>[2x]GIGDPVTCLKSGA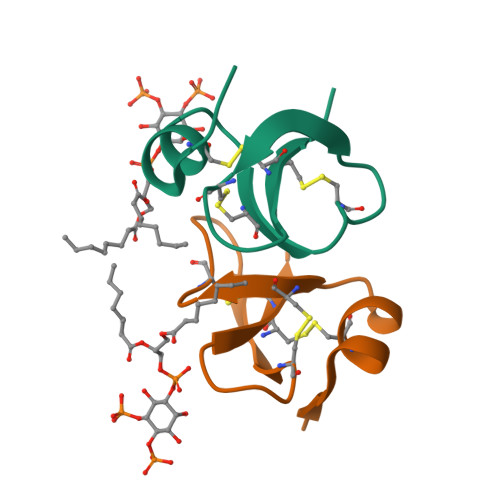ICHPVFCPRRYKQIGTCGLPGTKCCKKP> GPMAGAATQASLESAPRIMRLVAECSRSRARAGELWLPHGTVATPVFMPVGTQATMKGITTEQLDALGCRICLGNTYHLGLRPGPELIQKANGLHGFMNWPHNLLTDSGGFQMVSLVSLSEVTEEGVRFRSPYDGNETLLSPEKSVQIQNALGSDIIMQLDDVVSSTVTGPRVEEAMYRSIRWLDRCIAAHQRPDKQNLFAIIQGGLDADLRATCLEEMTKRDVPGFAIGGLSGGESKSQFWRMVALSTSRLPKDKPRYLMGVGYATDLVVCVALGCDMFDCVFPTRTARFGSALVPTGNLQLRKKVFEKDFGPIDPECTCPTCQKHSRAFLHALLHSDNTAA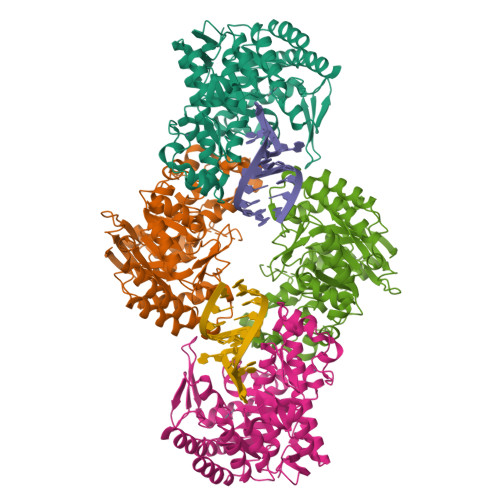LHHLTVHNIAYQLQLMSAVRTSIVEKRFPDFVRDFMGAMYGDPTLCPTWATDALASVGITLG;> MKLSLTKVVNGCRLGKIKNLGKTGDHTMDIPGCLLYTKTGSAPHLTHHTLHNIHGVPAMAQLTLSSLAEHHEVLTEYKEGVGKFIGMPESLLYCSLHDPVSPCPAGYVTNKSVSVWSVAGRVEMTVSKFMAIQKALQPDWFQCLSDGEVSCKEATSIKRVRKSVDRSLLFLDNCLRLQEESEVLQKSVIIGVIEGGDVMEERLRSARETAKRPVGGFLLDGFQGNPTTLEARLRLLSSVTAELPEDKPRLISGVSRPDEVLECIERGVDLFESFFPYQVTERGCALTFSFDYQPNPEETLLQQNGTQEEIKCMDQIKKIETTGCNQEITSFEINLKEKKYQEDFNPLVRGCSCYCCKNHTRAYIHHLLVTNELLAGVLLMMHNFEHYFGFFHYIREALKSDKLAQLKELIHRQAS>SMNPIEDDLIFRVGTKGRNKGEFTNLQGVAASTNGKILIADSNNQCVQIFSNDGQFKSRFGIRGRSPGQLQRPTGVAVHPSGDIIIADYDNKWVSIFSSDGKFKTKIGSGKLMGPKGVSVDRNGHIIVVDNKACCVFIFQPNGKIVTRFGSRGNGDRQFAGPHFAAVNSNNEIIITDFHNHSVKVFNQEGEFMLKFGSNGEGNGQFNAPTGVAVDSNGNIIVADWGNSRIQVFDGSGSFLSYINTSADPLYGPQGLALTSDGHVVVADSGNHCFKVYRYLQ[4x]

Tripartite motif (TRIM) proteins constitute one of the largest subfamilies of the RING-type E3 ubiquitin ligases that play a role in diverse processes from homeostasis and immune response to viral restriction. The NHL domain, or so-called NHL repeats named after ncl-1, HT2A and lin-41, forms another protein module found in four TRIMs, including TRIM2, TRIM3, TRIM32 and TRIM71, that constitute the subclass VII. Here, high-resolution crystal structures of the NHL domains of three of the four human TRIM–NHL proteins, namely TRIM2, TRIM3 and TRIM71, are presented. Comparative structural analyses revealed that, despite sharing an evolutionarily conserved six-bladed β-propeller architecture, the low sequence identities resulted in distinct properties of these interaction domains at their putative binding sites for macromolecules.

The NHL domains of TRIM2 and TRIM3 were highly expressed as a fusion protein with an N-terminal His6-GST tag in E. coli. For TRIM2, the structure was refined to a high resolution of 1.45 Å, and the crystals belonged to the monoclinic P21 space group with four molecules in the asymmetric unit. Nonetheless, an exception was noted when comparing TRIM2 and TRIM3 that were most similar with ∼82% sequence identity. In contrast, the rather shallow flat surface of the TRIM2/3 NHLs resembles that of their homologue DmBrat, which has been shown to recognize a linear RNA. However, comparative analyses suggest that similar binding of an RNA observed previously in DmBrat would be unlikely in TRIM2/3 due to the lack of a central channel as well as low sequence conservation within the pockets. TRIM2 NHL has been shown to interact with the motor-protein myosin V, and the function of this E3 ligase has been linked to neuronal activity including neurons and axon growth. In line with this, genetic studies have unveiled a number of mutations in the NHL motifs of TRIMs with a link to diverse pathological outcomes, in particular, diverse neurological disorders. This includes a link of the mutations in TRIM2 NHL to Charcot-Marie-Tooth disease (CMT), congenital bilateral vocal-cord paralysis (BVCP) and axonal neuropathy. A frameshift within blade 2 (K567Rfs7X) undoubtedly leads to a loss of the NHL domain, whereas the other nonsense mutation (R741X) results in the loss of four amino acids at the C terminus on the bottom surface. The other mutations include a substitution, D640A, and a deletion, N594del, both of which are located in the proximity of the central groove on the top surface, thus they could affect directly the integrity of the intermolecular interface.> MGHHHHHHAENLYFQGADPFESYNPEFFLYDIFLKFCLKYIDGEICHDLFLLLGKYNILPYDTSNDSIYACTNIKHLDFINPFGVAAGFDKNGVCIDSILKLGFSFIEIGTITPRGQTGNAKPRIFRDVESRSIINSCGFNNMGCDKVTENLILFRKRQEEDKLLSKHIVGVSIGKNKDTVNIVDDLKYCINKIGRYADYIAINVSSPNTPGLRDNQEAGKLKNIILSVKEEIDNLEKNNIMNDESTYNEDNKIVEKKNNFNKNNSHM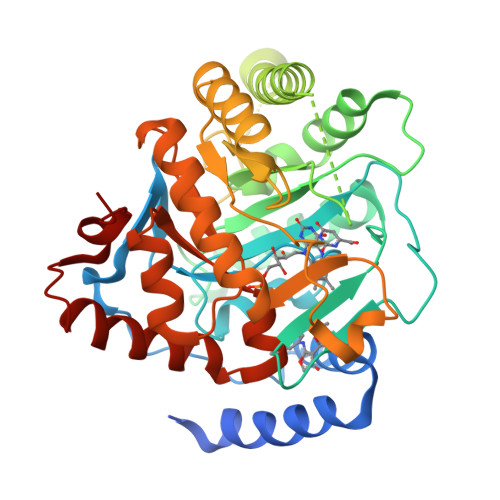MKDAKDNFLWFNTTKKKPLVFVKLAPDLNQEQKKEIADVLLETNIDGMIISNTTTQINDIKSFENKKGGVSGAKLKDISTKFICEMYNYTNKQIPIIASGGIFSGLDALEKIEAGASVCQLYSCLVFNGMKSAVQIKRELNHLLYQRGYYNLKEAIGRKHSKS> GTFTWTLSDSEGKDTPGGYCLTRWMLIEAELKCFGNTAVAKCNEKHDEEFCDMLRLFDFNKQAIQRLKAEAQMSIQLINKAVNALINDQLIMKNHLRDIMGIPYCNYSKYWYLNHTTTGRTSLPKCWLVSNGSYLNETHFSDDIEQQADNMITEMLQKEYMERQGKTPLGLVDLFVFSTSFYLISIFLHLVKI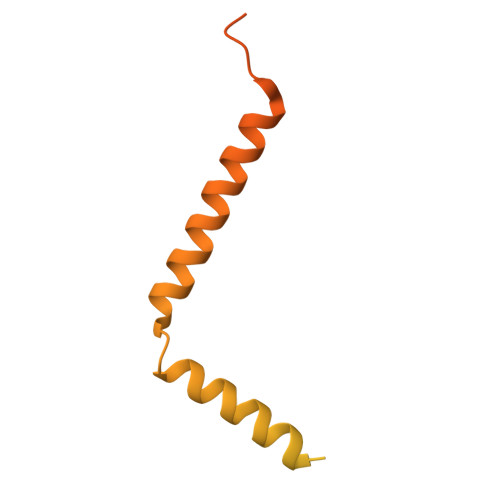PTHRHIVGKSCPKPHRLNHMGICSCGLYKQPGVPVKWKR>[2x]MGGSVIVIDSKAAWDAQLAKGKEEHKPIVVDFTATWSGPCKMIAPLFETLSNDYAGKVIFLKVDVDAVAAVAEAAGITAMPTFHVYKDGVKADDLVGASQDKLKALVAKHAAA

Thioredoxins (TRXs) are small oxidoreductases that contribute, in most living organisms, to the control of cellular redox homeostasis. Indeed, they reduce disulfide bonds on numerous proteins involved in several processes, including antioxidant defense mechanisms, photosynthetic carbon metabolism, and protein folding. In addition, TRXs have been suggested to control two additional Cys-based post-translational modifications, namely S-glutathionylation and S-nitrosylation, by catalyzing the reduction of glutathione-mixed disulfides (–SSGs) and S-nitrosothiols (–SNOs), respectively. The redox activity of TRXs relies on the presence of two Cys residues in the conserved Trp-Cys-(Gly/Pro)-Pro-Cys (WC(G/P)PC) active site motif.

In the present study, we deepen the structural features of CrTRXh1, providing the 3D structures of both the reduced form and variants in which catalytic cysteines were mutated. Regardless of the reducing activity in which TRXs are involved, the N-terminal active site Cys (CysN) is responsible for the first nucleophilic attack on oxidized targets. While the subsequent catalytic steps underlying TRX-dependent protein deglutathionylation and denitrosylation are yet undefined, the reduction of protein disulfides implies the formation of a mixed-disulfide bond between the CysN and a Cys on target protein.>[4x]MKILKTLTLRGPNYWSIRRKKLIVMRLDLEDLAERPSNSIPGFYEGLIKVLPSLVEHFCSPGYQGGFLERVKEGTYMGHIVEHVALELQELVGMTAGFGRTRETSTPGVYNVVYEYVDEQAGRYAGRAAVRLCRSLVDTGDYPRLELEKDLEDLRDLGANSALGPSTETIVTEAEARKIPWMLLSARAMVQLGYGVYQQRIQATLSSHSGILGVELACDKEGTKTILQDAGIPVPRGTTIQYFDDLEEAINDVGGYPVVIKPLDGNHGRGITINVRHWQEAIAAYDLAAEESKSRAIIVERYYEGSDHRVLVVNGKLVAVAERIPAHVTGDGSSTISELIEKTNQDPNRGDGHDNILTKIVVNKTAIDVMERQGYNLDSVLP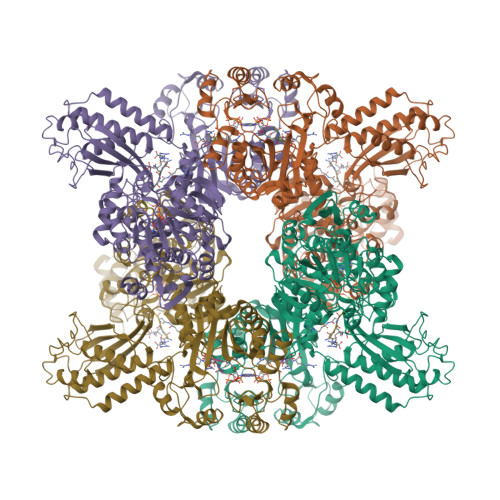KDEVVYLRATANLSTGGIAIDRTDDIHPENIWLMERVAKVIGLDIAGIDVVTSDISKPLRETNGVIVEVNAAPGFRMHVAPSQGLPRNVAAPVLDMLFPPGTPSRIPILAVTGTNGKTTTTRLLAHIYRQTGKTVGYTSTDAIYINEYCVEKGDNTGPQSAGVILRDPTVEVAVLETARGGILRAGLAFDSCDVGVVLNVAADHLGLGDIDTIEQMAKVKSVIAEVVDPSGYAVLNADDPLVAAMADKVKAKVAYFSMNPDNPIIQAHVRRNGIAAVYESGYLSILEGSWTLRVEQAKLIPMTMGGMAPFMIANALAACLAAFVNGLDVEVIRQGVRTFTTSAEQTPGRMNLFNLGQHHALVDYAHNPAGYRAVGDFVKNWQGQRFGVVGGPGDRRDSDLIELGQIAAQVFDRIIVKEDDDKRGRSEGETADLIVKGILQENPGASYEVILDETIALNKALDQVEEKGLVVVFPESVTRAIDLIKVRNPIGENLYFQ;>[8x]DDDDDDDDN>MKTIIINGVQFNTDEDTTILKFARDNNIDISALCFLNNCNNDINKCEICTVEVEGTGLVTACDTLIEDGMIINTNSDAVNEKIKSRISQLLDIHEFKCGPCNRRENCEFLKLVIKYKARASKPFLPKDKTEYVDERSKSLTVDRTKCLLCGRCVNACGKNTETYAMKFLNKNGKTIIGAEDEKCFDDTNCLLCGQCIIACPVAALSEKSHMDRVKNALNAPEKHVIVAMAPSVRASIGELFNMGFGVDVTGKIYTALRQLGFDKIFDINFGADMTIMEEATDLVQRIENNGPFPMFTSCCPGWVRQAENYYPELLNNLSSAKSPQQIFGTASKTYYPSISGLDPKNVFTVTVMPCTSKKFEADRPQMEKD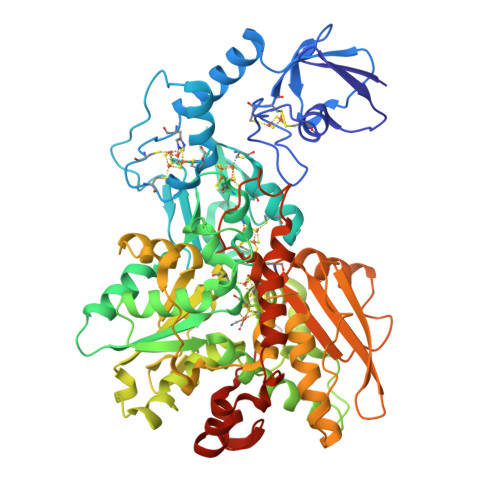GLRDIDAVITTRELAKMIKDAKIPFAKLEDSEADPAMGEYSGAGAIFGATGGVMEAALRSAKDFAENAELEDIEYKQVRGLNGIKEAEVEINNNKYNVAVINGASNLFKFMKSGMINEKQYHFIEVMACHGGCVNGGGQPHVNPKDLEKVDIKKVRASVLYNQDEHLSKRKSHENTALVKMYQNYFGKPGEGRAHEILHFKYKKSAWSHPQFEK[2x]> IVGGTDATLGEFPYQLSFQETFIGFSFHFCGASIYNENYAITAGHCVYGDDYENPS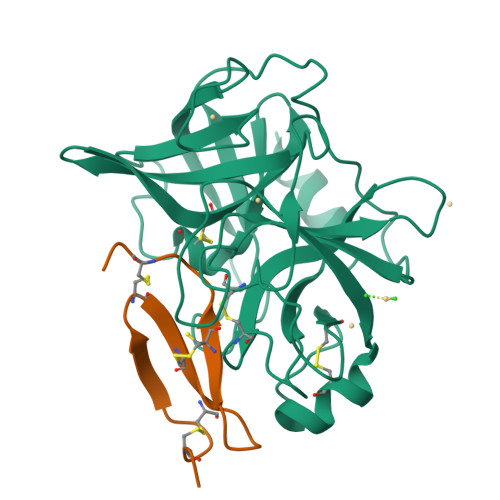GLQIVAGELDMSVNEGSEQIITVSKIILHENFDYNLLDNDISLLKLSGSLTFNDNVAPIALPEQGHTATGDVIVTGWGTTSEGGNTPDVLQKVTVPLVSDEDCRADYGADEILDSMICAGVPEGGKDSCQGDSGGPLAASDTGSTYLAGIVSWGYGCARPGYPGVYTEVSYHVDWIKANAV;> EQECTPGQTKKQDCNTCNCTPTGVWACTRKGCPPH>HHHHHHLEVLFQGPMKYTKLEKDALDLLSDNEEEDAESSILTFEERDTSSLSIEARLESIEEKLSMILGLLRTLNIATAGPTAARDGIRDAMIGVREELIADIIKEAKGKAAEMMEEE[8x]

The essential polymerase cofactor P from Pneumoviridae is a multifunctional hub which interacts with numerous components of the viral RNA-synthesis machinery. Pneumoviral P interacts with both L and the nucleocapsid, thereby tethering the polymerase to its template. In HMPV and RSV a central oligomerization domain facilitates the formation of P tetramers. In summary, we have shown that HMPV P is a highly dynamic protein that is composed of a stable helical tetramerization domain flanked by large N-terminal and C-terminal IDRs that sample a large volume in solution and display varying degrees of preformed structural elements.

Although we were not able to grow crystals of a complex, crystals which later proved to harbour only the P oligomerization region could be obtained after extended time periods. Serendipitously, we obtained two additional crystal forms of Pcore with improved resolution, allowing us to build a higher quality model (100% Ramachandran favoured). The first crystal (form 1, space group P21) diffracted to a resolution of 1.6 Å, while the second crystal (form 2, space group P212121) gave rise to diffraction data up to 2.2 Å. The P21 crystal (form 1) of HMPV Pcore grew at 20 °C after 291–344 days with mother liquor containing 20% polyethylene glycol (PEG) 6000, 200 mM NaCl, and 100 mM Tris, pH 8.0. Diffraction data were recorded on beamlines I03 (P21 crystal) and I04 (P212121 crystal) at Diamond Light Source, Didcot, UK. For the 1.6 Å data of crystal form 1 we additionally carried out anisotropic atomic displacement parameter (ADP) refinement. Mapping of the sequence conservation within the Pneumoviridae onto Pcore reveals the strict conservation of the hydrophobic amino acids (Leu and Ile residues) lining the interior of the coiled-coil, indicating that all family members share a similar P oligomerization region (strictly conserved residues in purple). Furthermore, Arg175 is strictly conserved in all Pneumoviridae and plays a role in stabilizing the quaternary structure of the tetramer by forming a salt bridge with either an Asp or Glu on the neighbouring helix. Alignment of all six tetramers from crystal forms 1 and 2 and the original crystal confirmed that there are small-scale breathing motions within the coiled-coil. The ability of the C-terminal region of P to stabilize this α-helical structure might explain its absence from the crystal structures of Pcore (as the P constructs used for crystallization required C-terminal degradation in order to yield diffracting crystals, which in turn destabilizes the cap-like structure).>MELNYDRLVQQTESWLPIVLEYSGKVALALLTLAIGWWLINTLTGRVGGLLARRSVDRTLQGFVGSLVSIVLKILLVVSVASMIGIQTTSFVAAIGAAGLAIGLALQGSLANFAGGVLILL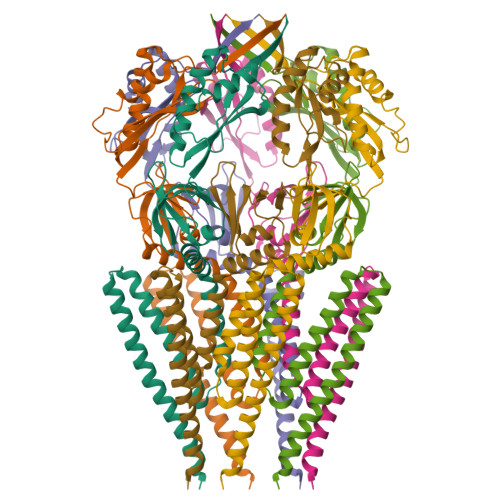FRPFKVGDWIEAQGVAGTVDSILIFHTVLRSGDNKRIIVPNGALSNGTVTNYSAEPVRRVIFDVGIDYDADLKNAQNILLAMADDPRVLKDPAPVAVVSNLGESAITLSLRVWVKNADYWDVMFMFNEKARDALGKEGIGIPFPQRVVKVVQGAMAD[7x]> MTIPFDHWPEWPQHSDRTRRKIEEVFQSNRWAI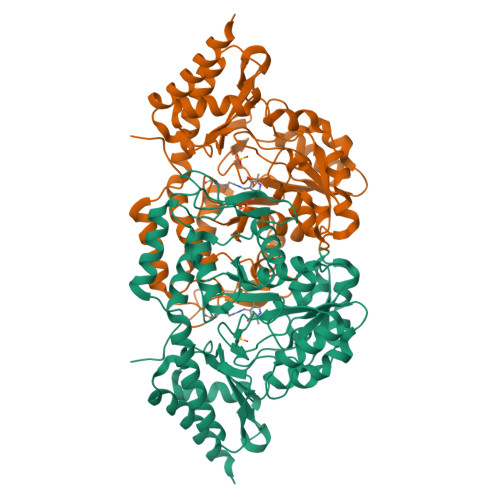SGYWTGEESMERKFAKAFADFNGVPYCVPTTSGSTALMLALEALGIGEGDEVIVPSLTWIATATAVLNVNALPVFVDVEADTYCIDPQLIKSAITDKTKAIIPVHLFGSMANMDEINEIAQEHNLFVIEDCAQSHGSVWNNQRAGTIGDIGAFSCQQGKVLTAGEGGIIVTKNPRLFELIQQLRADSRVYCDDSSELMHGDMQLVKKGDIQGSNYCLSEFQSAILLDQLQELDDKNAIREKNAMFLNDALSKIDGIKVMKRPPQVSRQTYYGYVFRFDPVKFGGLNADQFCEILREKLNMGTFYLHPPYLPVHKNPLFCPWTKNRYLKSVRKTEAYWRGLHYPVSERASGQSIVIHHAILLAEPSHLSLLVDAVAELARKFCVTH>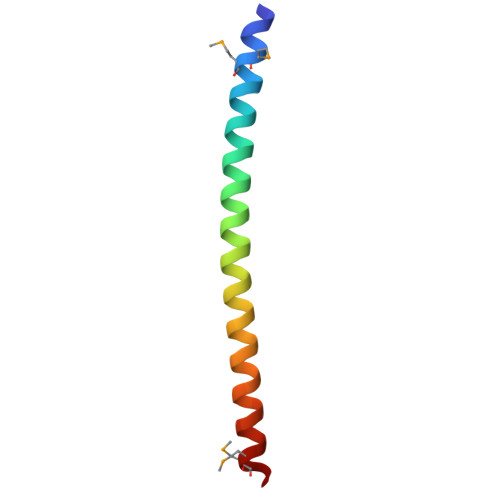 SDDDIMMYESAELKRVEEEIEELKRKILVRKKHDLRKLSLNNQLQELQSMMDG>[8x]HMTDGERQNATEIRASVGKMIDGIGRFYIQMCTELKLSDYEGRLIQNSLTIERMVLSAFDERRNKYLEEHPSAGKDPKKTGGPIYRRVDGKWRRELILYDKEEIRRIWRQANNGDDATAGLTHMMIWHSNLNDATYQRTRALVRTGMDPRMCSLMQGSTLPRRSGAAGAAVKGVGTMVMELIRMIKRGINDRNFWRGENGRRTRIAYERMCNILKGKFQTAAQRTMVDQVRESRNPGNAEFEDLI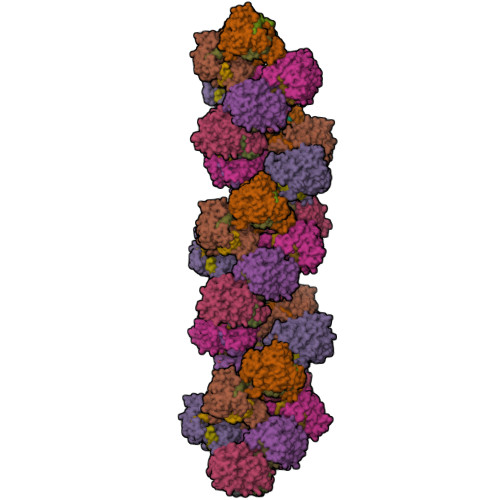FLARSALILRGSVAHKSCLPACVYGSAVASGYDFEREGYSLVGIDPFRLLQNSQVYSLIRPNENPAHKSQLVWMACHSAAFEDLRVSSFIRGTKVVPRGKLSTRGVQIASNENMETMESSTLELRSRYWAIRTRSGGNTNQQRASSGQISIQPTFSVQRNLPFDRPTIMAAFTGNTEGRTSDMRTEIIRLMESARPEDVSFQGRGVFELSDEKATSPIVPSFDMSNEGSYFFGDNAEEYDNLEHHHHHH> MVDSIVEGRTLNVAVSPASPPMLFKSADGKL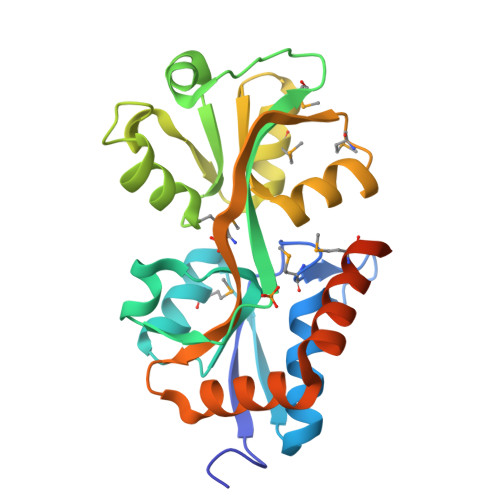QGIDLELFSSYCQSRHCKLNITEYAWDGMLGAVASGQADVAFSGISITDKRKKVIDFSEPYYINSFYLVSMANHKITLNNLNELNKYSIGYPRGMAYSDLIKNDLEPKGYYSLSKVKLYPTYNETMADLKNGNLDLAFIEEPVYFTFKNKKKMPIESRYVFKNVDQLGIAFKKGSPVRDDFNLWLKEQGPQKISGIVDSWMKAENLYFQSHHHHHHWSHPQFEK A glucosylglycerate hydrolase (GgH) identified in M. hassiacum and found to be highly conserved among rapidly growing mycobacteria is likely to be responsible for the rapid mobilization of GG accumulated during nitrogen starvation by hydrolysing it to glucose and glycerate. The MhGgH monomer displays an (α/α)6-barrel domain typical of glycoside hydrolase family 63 (GH63), to which MhGgH belongs. While the active site of GH63 members acting on larger substrates is located in an open, solvent-accessible cleft, those of MhGgH and of MgH from T. thermophilus are covered by a cap domain (subdivided into A′- and B′-regions) with constrained access through a narrow negatively charged tunnel. The crystallographic structure of MhGgH revealed a homotetrameric architecture, which is compatible with the oligomeric organization of the enzyme in solution as assessed by SAXS.

In an alternative crystallization condition (space group P6222), two MhGgH protomers are present in the asymmetric unit, corresponding to molecules A and C of the tetramer observed in the orthorhombic crystals, which were modelled from Pro5 (molecule A) or Ala0 (molecule C) to Gly446. The active sites of both molecules contain only solvent (apo MhGgH) and adopt an open conformation. In contrast to the closed conformation, the putative catalytic residues point away from the active-site cavity: Asp182 is stabilized by polar contacts with the side chains of Tyr191 and Tyr225 and with the carbonyl group of Arg216 through a water molecule, whereas the side chain of Glu419 is hydrogen-bonded to the side chain of Ser435 and the amide N atoms of Met432 and Thr437. The two structures of MhGgH, apo MhGgH and MhGgH–Ser–GOL, corresponding to its open and closed conformations, reveal the structural modifications that occur upon substrate binding. In the open conformation, Gln433 and Gln434 move outwards (with displacements of their side chains of ∼11 and ∼8 Å, respectively), leading to a concerted rearrangement of loop E and loop A. Loop A (Arg21–Ala31) becomes mostly disordered, with difficult-to-interpret density that only allowed the modelling of two conformations for the segment Leu20–Leu25. In this short stretch, the contribution of Asp24-mediated interactions (with Arg21 or Arg58 of the neighbouring molecule) appears to be central to the overall conformation of this region. Moreover, given their spatial proximity, the conformation adopted by one subunit determines the position of the equivalent region of the neighbouring molecule, potentially impacting enzyme activity, which is in good agreement with the cooperative behaviour observed in the kinetics experiments [Fig. 1(c)].

>[2x]GAMPHDPSFTPTQLAARAAYLLRGNDLGTMTTAAPLLYPHMWSWDAAFVAIGLAPLSVERAVVELDTLLSAQWRNGMIPHIVFANGVDGYFPGPARWATATLADNAPRNRLTSGITQPPVHAIAVQRILEHARTRGRSTRAVAEAFLDRRWGDLMRWHRWLAECRDRNERGRITLYHGWESGMDNSPRWDSAYANVVPGKLPEYQRADNVIITDPSQRPSDGEYDRYLWLLEEMKAVRYDDERLPSVMSFQVEDVFFSAIFSVACQVLAEIGEDYKRPHADVKDLYLWAERFRAGVVETTDQRTGAARDFDVLAEKWLVTETAAQFAPLLCGGLPHDRERALLKLLEGPRFCGHPDLKYGLIPSTSPVSRDFRPREYWRGPVWPVLTWLFSWCFARRGWAERARLLRQEGLRQASDGSFAEYYEPFTGEPLGSMQQSWTAAAVLDWLG> ANGQSTRYWDCCKPSCGWRGKGPVNQPVYSCDANFQRIHDFDAVSGCEGGPAFSCADHSPWAINDNLSYGFAATALSGQTEESWCCACYA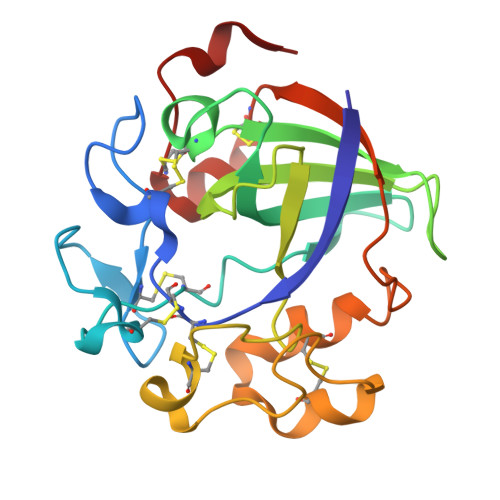LTFTSGPVAGKTMVVQSTSTGGDLGSNHFDLNIPGGGVGLFDGCTPQFGGLPGARYGGISSRQECDSFPEPLKPGCQWRFDWFQNADNPSFTFERVQCPEELVARTGCRRHDDGGFA>MEKSNRSLKDLDLNALFIGDKAENGQLYKDLLNKLVDEHLGWRKNYIPSDPNMIGPEDQNSPAFKKTVGHMKTVLDQLSERIRTESVPWHSAGRYWGHMNSETLMPALLAYNYAMLWNGNNVAYESSPATSQMEEEVGQEFARLMGYDYGWGHIVADGSLANLEGLWYARNIKSLPFAMKEVNPELVAGKSDWELLNMPTKEIMDLLENAGSQIDEVKKRSARSGKNLQRLGKWLVPQTKHYSWMKAADIIGIGLDQVVPVPIDSNYRMDIQALESIIRKYAAEKTPILGVVGVAGSTEEGAVDGIDKIVALRQKLQKEGIYFYLHVDAAYGGYARALFLDEDDQFIPYKNLQKVHAENHVFTEDKEYIKPEVYAAYKAFDQAESITIDPHKMGYVPYSAGGIVIQDIRMRDTISYFATYVFEKGADIPALLGAYILEGSKAGATAASVWAAHHTLPLNVTGYGKLEGASIEGAHRYYDFLKNLKFEVAGKRISVHPLISPDFNMVDYVLKEDGNDDLIEMNRLNHAFYEQASYVKGSLYGKEYIVSHTDFAIPDYGDSPLAFVESLGFSEVEWRHAGKVTIIRASVMTPYMNQRENFDYFAPRIKKAIQADLEKVYASVNQKENVLEHHHHHH[2x]

Tyrosine decarboxylase (TDC, EC 4.1.1.25) is classified into Group II and shares high identity with L-3,4-dihydroxy-L-phenylalanine (DOPA) decarboxylase (DDC), glutamic acid decarboxylase (GAD), and histidine decarboxylase (HDC). TDC could catalyze the decarboxylation of L-tyrosine and L-DOPA to tyramine and dopamine. LbTDC is a homodimer, and the two subunits exist in an asymmetric form. Similar to the structures of other Group II decarboxylases, each LbTDC monomer is composed of three distinct domains: the N-terminal (residues 7–105) domain, the PLP-binding (residues 106–462) domain, and the small (residues 463–618) domain.

After optimization of the crystallization conditions, the crystals of LbTDC alone and in complex with PLP (apo-LbTDC and holo-LbTDC, respectively) were obtained and the corresponding three-dimensional structures were resolved. Compared with the open conformation of the apo form of the human DDC structure, the structure of apo-LbTDC is in a closed conformation. A comparison of the structure of apo-LbTDC with the structure of holo-LbTDC revealed that there are two opposite conformations of K240 and H241. In the apo-LbTDC structure, the imidazole ring of H241 is anchored by two water molecules and is distant from the PLP binding pocket, and the side chain of K240 is placed in a position near the PLP binding pocket. Residues K240 and H241 form a short flexible loop. Additionally, through a structural alignment with drDDC and pig DDC, a conserved histidine (H192) was also identified, which has been reported to interact with the pyridine ring of PLP. This interesting dynamic change in conformation suggests that K240 and H241 play important roles in establishing the conformation required for the binding and stabilization of cofactor and substrate.>MNPTIIRARAPLRLGLAGGGTDVAPYADTFGGYVLNATIDRYAYAVIKTLTIPAVRFVST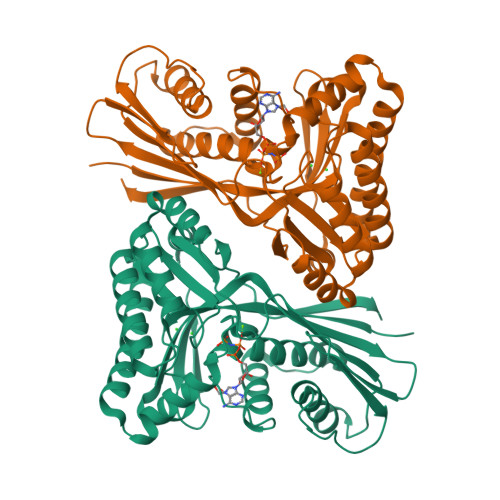DQQVEKHQLISEPLELNGTLNLHKAVYNHMIRNYNHGKPIALELSTFCDAPAGSGLGSSSTLVVVMIKAFVELLNLPLDDYAIAQLAYRIERVDCGLAGGRQDQYSATFGGFNFMEFYAAARTIVNPLRIKNWVLCELEASLVLFYTGVSRESAKIIQDQSDNVVSHKTAAIEAMHGIKREALVMKEALLKGDFKAFVASMRLGWDNKKNSARTVSNAHIDEIYDAAIRAGAQAGKVSGAGGGGFMLFFVPTEKRMDLIRTLGEYDGQVSNCHFTKNGTQAWRIAN[2x]> DDYLWGLEAGEGIS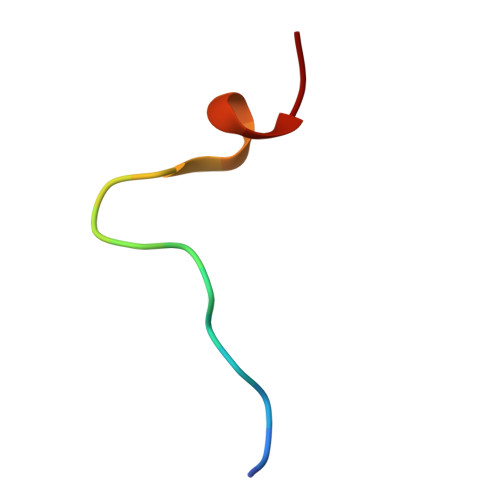DLFD> MARRKCRNRFVKKNGQCNVEFTNMDDKPQRYIADMFTTCVDIRWRYMLLLFSLAFLVSWLLFGLIFWLIALIHGDLENPGGDDTFKPCVLQVNGFVAAFLFSIETQTTIGYGFRCVTEECPLAVFMVVVQSIVGCIIDSFMIGAIMAKMARPKKRAQTLLFSHNAVV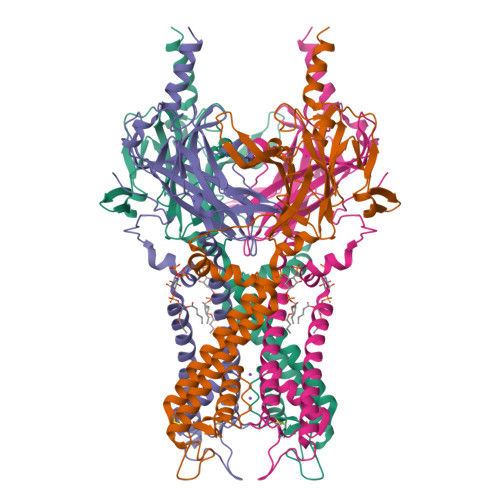AMRDGKLCLMWRVGNLRKSHLVEAHVRAQLIKPRITEEGEYIPLDQIDIDVGFDKGLDRIFLVSPITILHEINEDSPLFGISRQDLETDDFEIVVILEGMVEATAMTTQARSSYLASEILWGHRFEPVLFEEKNQYKVDYSHFHKTYEVPSTPRCSAKDLVENKFLLSNSLEVLFQ>MAQVINTNSLSLITQNNINKNQSALSSSIERLSSGLRINSAKDDAAGQAIANRFTSNIKGLTQAARNANDGISVAQTTEGALSEINNNLQRIRELTVQATTGTNSDSDLDSIQDEIKSRLDEIDRVSGQTQFNGVNVLAKDGSMKIQVGANDGETITIDLKKIDSDTLGLNGFNVNGKGTITNKAATVSDLTSAGAKLNTTTGLYDLKTENTLLTTDAAFDKLGNGDKVTVGGVDYTYNAKSGDFTTTKSTAGTGVDAAAQAADSASKRDALAATLHADVGKSVNGSYTTKDGTVSFETDSAGNITIGGSQAYVDDAGNLTTNNAGSAAKADMKALLKAASEGSDGASLTFNGTEYTIAKATPATTTPVAPLIPGGITYQATVSKDVVLSETKAAAATSSITFNSGVLSKTIGFTAGESSDAAKSYVDDKGGITNVADYTVSYSVNKDNGSVTVAGYASATDTNKDYAPAIGTAVNVNSAGKITTETTSAGSATTNPLAALDDAISSIDKFRSSLGAIQNRLDSAVTNLNNTTTNL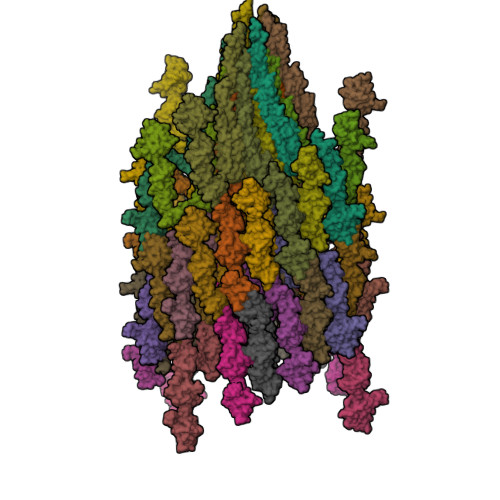SEAQSRIQDADYATEVSNMSKAQIIQQAGNSVLAKANQVPQQVLSLLQG[44x]> MLDAFSRVVTNADSKAAYVGGADLQALKKFISEGNKRLDSVNSIVSNASCI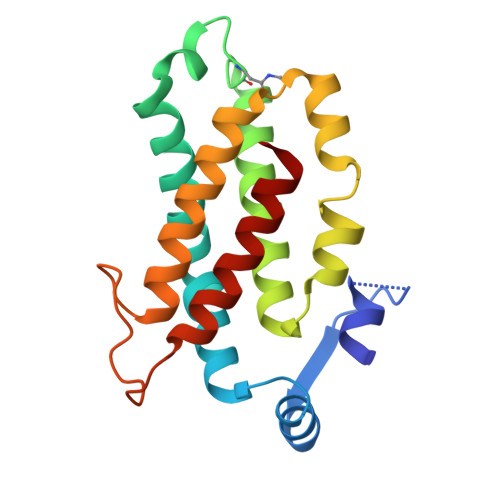VSDAVSGMICENPSLISPSGNCYTNRRMAACLRDGEIILRYVSYALLSGDASVLEDRCLNGLKETYSSLGVPANSNARAVSIMKACAVAFVNNTASQKKLSTPQGDCSGLASEVGGYFDKVTAAIS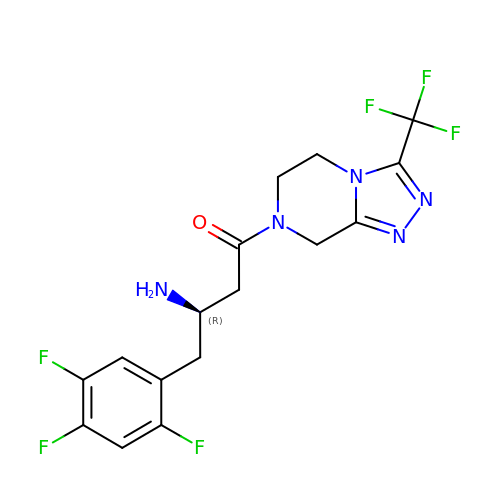(2R)-4-OXO-4-[3-(TRIFLUOROMETHYL)-5,6-DIHYDRO[1,2,4]TRIAZOLO[4,3-A]PYRAZIN-7(8H)-YL]-1-(2,4,5-TRIFLUOROPHENYL)BUTAN-2-AMINE | C16 H15 F6 N5 O | MFFMDFFZMYYVKS-SECBINFHSA-N>[5x]SNAMKIGIIGVGKMASAIIKGLKQTPHELIISGSSLERSKEIAEQLALPYAMSHQDLIDQVDLVILGIKPQLFETVLKPL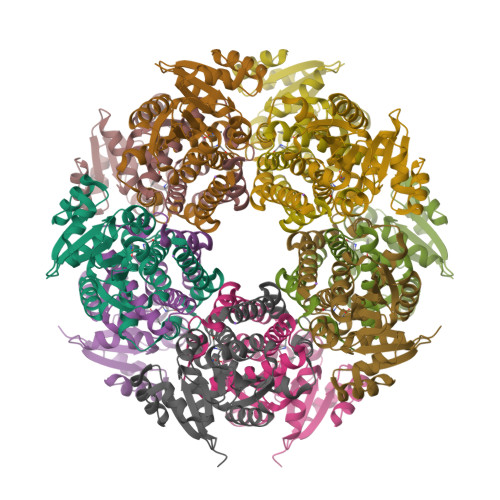HFKQPIISMAAGISLQRLATFVGQDLPLLRIMPNMNAQILQSSTALTGNALVSQELQARVRDLTDSFGSTFDISEKDFDTFTALAGSSPAYIYLFIEALAKAGVKNGIPKAKALEIVTQTVLASASNLKTSSQSPHDFIDAICSPGGTTIAGLMELERLGLTATVSSAIDKTIDKAKSL> MESKKRQWALEDFEIGRPLGKGKFGNVYLAREKQSKFILALKVLFKAQLEKAGVEHQLRREVEIQSHLRHPNILRLYGYFHDATRVYLILEYAPLGTVYRELQKLSKFDEQRTATYITELANALSYCHSKRVIHRDIKPENLLLGSAGELKIANFGWSVHA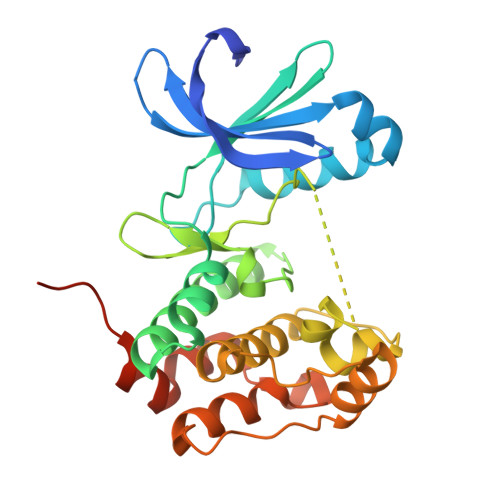PSSRRTTLAGTLDYLPPEMIEGRMHDEKVDLWSLGVLCYEFLVGKPPFEANTYQETYKRISRVEFTFPDFVTEGARDLISRLLKHNPSQRPMLREVLEHPWITANSSKPSNAQNKESASKQS>MNKSQLYPDSPLTDQDFNQLDQTVIEAARRQLVGRRFIELYGPLGRGMQSVFNDIFMESHEGGGEIQQLEEEIAQLEQKNAALKEKNQALKAGGGAKMDFQGSFDTEVESSRRVNYTIPMLYKDFVLYWRDLEQSKALDIPIDFSVAANAARDVAFLEDQMIFHGSKEFDIPGLMNVKGRLTHLIGNWYESGNAFQDIVEARNKLLEMNHNGPYALVLSPELYSLLHRVHKDTNVLEIEHVRELITAGVFQSPVLKGKSGVIVNTGRNNLDLAISEDFETAYLGEEGMNHPFRVYETVVLRIKRPAAICTLIDPEEHHH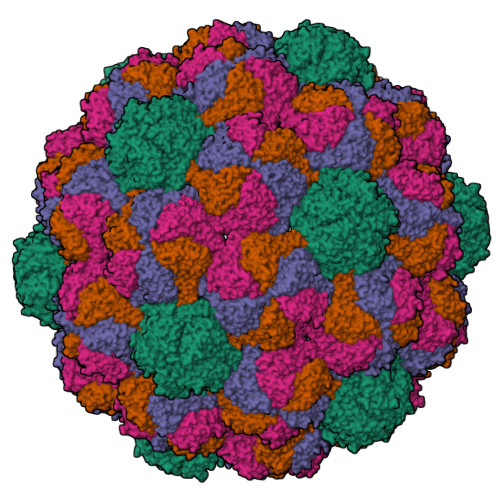HHHHH[4x]N-[4-[(5R)-1-(4-azanylbutyl)-6-oxidanylidene-5-quinolin-5-yl-4,5-dihydropyridazin-3-yl]phenyl]-1,3-dihydropyrrolo[3,4-c]pyridine-2-carboxamide 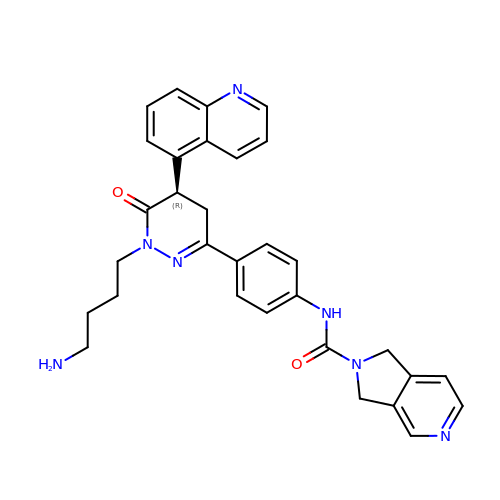| C31 H31 N7 O2 | NJFRNKQNKJTDFZ-HHHXNRCGSA-N1-(3-deoxy-3-fluoro-beta-D-glucopyranosyl)pyrimidine-2,4(1H,3H)-dione | 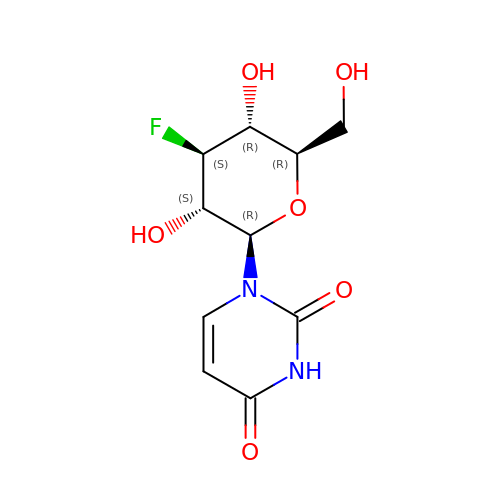C10 H13 F N2 O6 | QGWLQEMDCINRKW-PMPOVCSBSA-N> GPGSRSICSRHTRHGVDRSHFSLRDFFRGISANFELGKDFLREMNTPIHVSEAVFLPLSLCTLSPGRCLRLSPFGHSLTLGSHCEICINRSQVHVPQEFSSTQLSFFNNVHKIIPNKTFYVSLLSSSPSAVKAGLSQPSLLYAYLVTGHFCGTICPIFSTNGKGRLIMHLLLQGTSLHIPETCLKLLCENIGPTYEL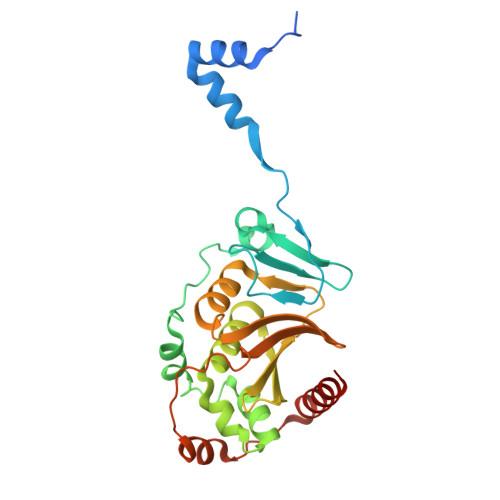AVDLVGDAFCIKVSPRDTVYEKAVNVDEDAIYEAIKDLECGDELRLQIINYTQLILENKQ CueO plays an important role in copper homeostasis by oxidation of toxic cuprous ions to cupric ions. As with all multi-copper oxidases, it contains four copper atoms distributed within one type 1 (T1)2 copper site and a trinuclear cluster comprising the T2 and T3 copper sites. A distinguishing feature of CueO is a partially structured 45-amino acid segment (residues 356–404) capping the entrance to the T1/sCu copper-binding sites. The goal of the current study was to engineer the highly compliant MRS such that CueO activity would be modulated by engagement of a partner protein with a scaffolded peptide.

A panel of CueO variants was generated with differing modifications in the MRS. These included insertion of the parental MDM2-binding peptide sequence present in the N-terminal domain of p53 along with a higher-affinity derivative (peptide 12.1) into the MRS α5 helix to generate CueO-p53 and CueO-12.1-α5, respectively. The results showed interaction with MDM2 only for the CueO-12.1 variant, where the 12.1 peptide replaced residues 384–394 in the intrinsically disordered region of the MRS. Kinetics data indicated that insertions into the MRS primarily affected kcat for syringaldazine oxidation, with no marked influence on affinity. This was most pronounced for the 12.1 and PM2 peptide insertions, reducing kcat ∼2.2- and 2.8-fold, respectively. To gain further mechanistic insights, we determined crystal structures of both the free and MDM2(6–125)-bound forms of CueO-PM2 along with CueO-12.1. However, in the highly similar structures of CueO-PM2 and CueO-12.1 (Cα RMSD = 0.22 Å), the MRS-PM2/12.1 regions were not resolved.

> AERPTLPIPDLLTTDARNRIQLTIGAGQSTFGGKTATTWGYNGNLLGPAVKLQRGKAVTVDIYNQLTEETTLHWHGLEVPGEVDGGPQGIIPPGGKRSVTLNVDQPAATCWFHPHQHGKTGRQVAMGLAGLVVIEDDEILKLMLPKQWGIDDVPVIVQDKKFSADGQIDYQLDVMTAAVGWFGDTLLTNGAIYPQHAAPRGWLRLRLLNGCNARSLNFATSDNRPLYVIASDGGLLPEPVKVSELPVLMGERFEVLVEVNDNKPFDLVTLPVSQMGMAIAPFDKPHPVMRIQPIAISASGALPDTLSSLPALPSLEGLTVRKLQLSMDPILDMMGMQMLMEKYGDQAMAGMDHSQMPRFMDYWEGLNMNHGGKFDFHHANKINGQAFDMNKPMFAAAKGQYERWVISGVGDMMLHPFHIHGTQFRILSENGKPPAAHRAGWKDTVKVEGNVSEVLVKFNHDAPKEHAYMAHCHLLEHEDTGMMLGFTVKDPNSSSVDKLAAALEHHHHHH> MNVDLVFLFDGSMSLQPDEFQKILDFMKDVMKKLSNTSYQFAAVQFSTSYKTEFD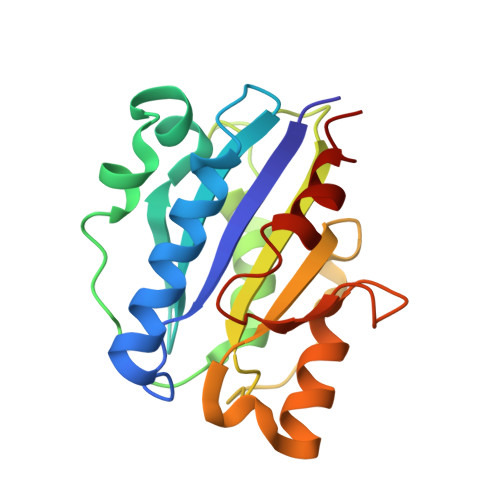FSDYVKWKDPDALLKHVKHMLLLTNTFGAINYVATEVFREELGARPDATKVLIIITDGEATDSGNIDAAKDIIRYIIGIGKHSQTKESQETLHKFASKPASEFVKILDTFEKLKDLFTELQKKIY>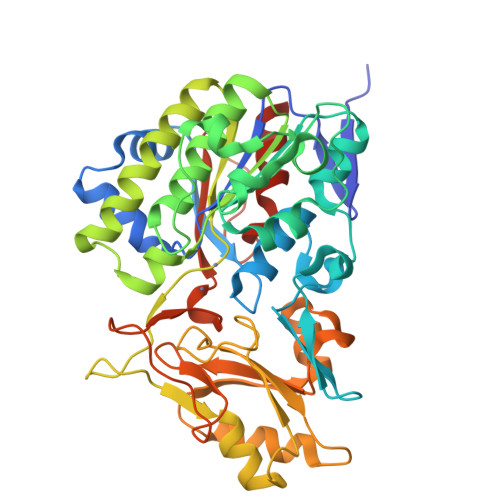 GSHMNQMSKISVTVNGRRYPWPRVPAIAVCLDGCEPAYLDAAIDAGLMPALKRIKERGAVRLAHSVIPSFTNPNNLSIATGSPPAVHGICGNYLYEPSTGEEVMMNDPKFLRAPTIFQAFYDAGARVAVVTAKDKLRALLGKGLRFDEGRAVCFSSEKSDKATRAEHGIDNASAWLGRPVPEVYSAALSEFVFAAGVKLLREFRPDIMYLTTTDYVQHKYAPGVPEANSFYEMFDRYLAELDGLGAAIVVTADHGMKPKHKADGSPDVIYVQDLLDEWLGKDAARVILPITDPYVVHHGALGSFATAYLPDGCDRSEIMARLKAIQGVDVVLGREEACRRFELPEDRIGDIVLVSSENKTLGTSEHRHDLAALDEPLRSHGGLTEQEVPFIVNRVLPELPNAPRLRNFDAFFYAVTAAAEAGAEGGL>GPTTFTIHTVESAPAEVKEILETVEKDNNGYIPNLIGLLANAPTVLEAYQIVSSIHRRNSLTPVEREVVQITAAVTNGCAFCVAGHTAFSIKQIQMNDDLIQALRNRTPIETDPKLDTLAKFTLAVINTKGRVGDEALSEFLEAGYTQQNALDVVFGVSLAILCNYANNLANTPINPELQPYA[6x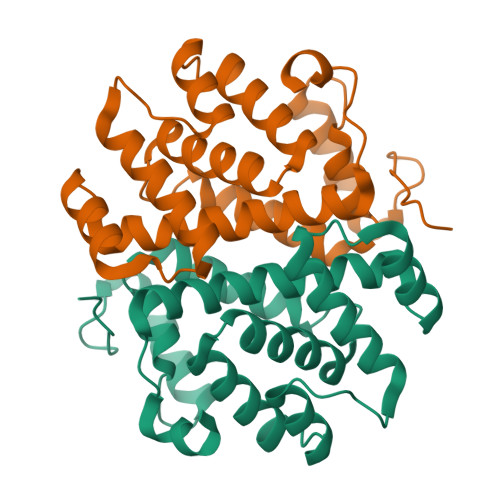]>[2x]MEGSEPVAAHQGEEASCSSWGTGSTNKNLPIMSTASVEIDDALYSRQRYVLGDTAMQKMAKSHVFLSGMGGLGLEIAKNLVLAGIKAVTIHDTEKCQAWDLGTNFFLSEDDVVNKRNRAEAVLKHIAELNPYVHVTSSSVPFNETTDLSFLDKYQCVVLTEMKLPLQKKINDFCRSQCPPIKFISADVHGIWSRLFCDFGDEFEVLDTTGEEPKEIFISNITQANPGIVTCLENHPHKLETGQFLTFREINGMTGLNGSIQQITVISPFSFSIGDTTELEPYLHGGIAVQVKTPKTVFFESLERQLKHPKCLIVDFSNPEAPLEIHTAMLALDQFQEKYSRKPNVGCQQDSEELLKLATSISETLEEKPDV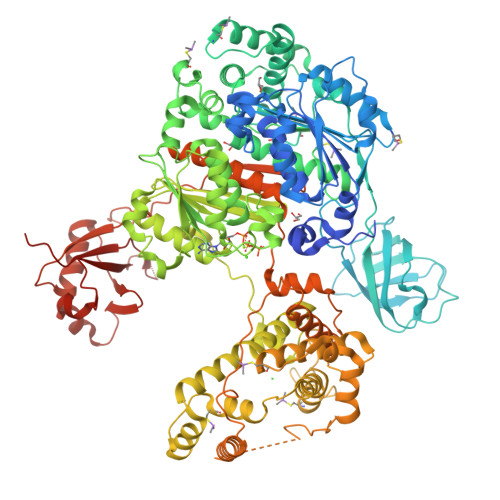NADIVHWLSWTAQGFLSPLAAAVGGVASQEVLKAVTGKFSPLCQWLYLEAADIVESLGKPECEEFLPRGDRYDALRACIGDTLCQKLQNLNIFLVGCGAIGCEMLKNFALLGVGTSKEKGMITVTDPDLIEKSNLNRQFLFRPHHIQKPKSYTAADATLKINSQIKIDAHLNKVCPTTETIYNDEFYTKQDVIITALDNVEARRYVDSRCLANLRPLLDSGTMGTKGHTEVIVPHLTESYNSHRDPPEEEIPFATLKSFPAAIEHTIQWARDKFESSFSHKPSLFNKFWQTYSSAEEVLQKIQSGHSLEGCFQVIKLLSRRPRNWSQCVELARLKFEKYFNHKALQLLHCFPLDIRLKDGSLFWQSPKRPPSPIKFDLNEPLHLSFLQNAAKLYATVYCIPFAEEDLSADALLNILSEVKIQEFKPSNKVVQTDETARKPDHVPISSEDERNAIFQLEKAILSNEATKSDLQMAVLSFEKDDDHNGHIDFITAASNLRAKMYSIEPADRFKTKRIAGKIIPAIATTTATVSGLVALEMIKVTGGYPFEAYKNCFLNLAIPIVVFTETTEVRKTKIRNGISFTIWDRWTVHGKEDFTLLDFINAVKEKYGIEPTMVVQGVKMLYVPVMPGHAKRLKLTMHKLVKPTTEKKYVDLTVSFAPDIDGDEDLPGPPVRYYFSHDTD>[4x]HHHHHHGSMALYGFAQGLIQEAGIRIKQLMEQNLTIETKSNPNDLVTNVDKATEDFIFDTILETYPNHQVLGEEGHGHDIDTSKGTVWVVDPIDGTLNFVHQQENFAISIGIYIDGKPYAGFVYDVMADVLYHAKVGEGAYRGSQPLKPLNDSNLRQSIIGINPNWLTKPILGEIFKEIVNDS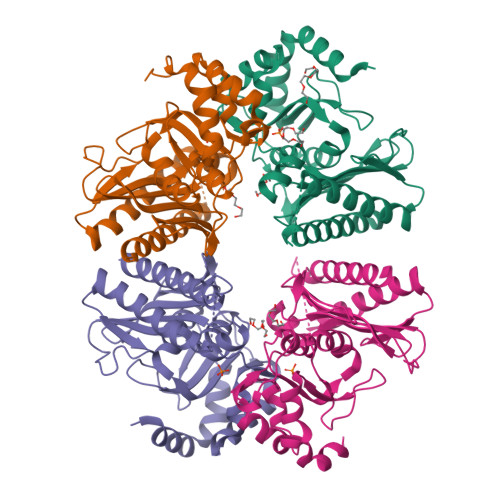RSARAYGSAALEIVSVATGNLEAYMTPRLQPWDFAGGLVILYEVNGQASNLLGEPLTISGPNSILVGNRGLHQEISNDYLEPHHDALIQLHEQRFKRKSK>[4x]MDIISVALKRHSTKAFDASKKLTAEEAEKIKTLLQYSPSSTNSQPWHFIVASTEEGKARVAKSAAG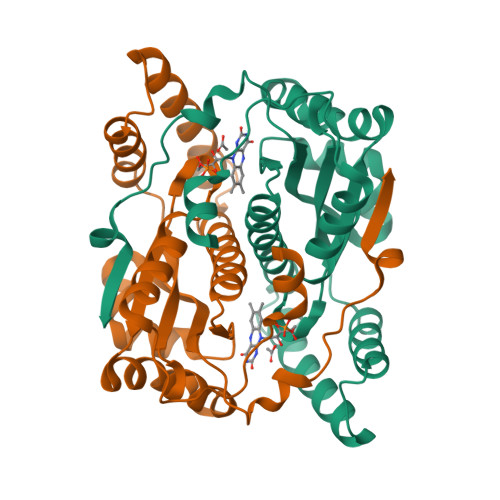TYVFNERKMLDASHVVVFCAKTAMDDAWLERVVDQEEADGRFNTPEAKAANHKGRTYFADMHRVDLKDDDQWMAKQVYLNVGNFLLGVGAMGLDAVPIEGFDAAILDEEFGLKEKGFTSLVVVPVGHHSVEDFNATLPKSRLPLSTIVTEC The versatile nucleotide excision repair (NER) pathway initiates as the XPC–RAD23B–CETN2 complex first recognizes DNA lesions from the genomic DNA and recruits the general transcription factor complex, TFIIH, for subsequent lesion verification. Here, we present a cryo-EM structure of an NER initiation complex containing Rad4–Rad23-Rad33 (yeast homologue of XPC–RAD23B–CETN2) and 7-subunit coreTFIIH assembled on a carcinogen-DNA adduct lesion at 3.9–9.2 Å resolution. The coreTFIIH contains two helicase-family ATPase subunits: XPB(Ssl2) and XPD(Rad3) in human(yeast), and 5 nonenzymatic subunits: p62(Tfb1), p52(Tfb2), p44(Ssl1), p34(Tfb4), and p8(Tfb5). Altogether, our study illustrates how the Rad4–Rad23–Rad33 (XPC–RAD23B–CETN2) complex recruits TFIIH to damaged DNA in 3D structural models and provides the groundwork to visualize how the NER initiation is carried out in multiple, coordinated yet distinct steps.

The most populated class resolved TFIIH at a nominal resolution of 3.86 Å, but with disordered density corresponding to the Rad4–Rad23–Rad33 complex bound to DNA (Map 1, EMDB-22587). Map 1 resolved TFIIH at a nominal resolution of 3.86 Å, the highest resolution for yeast TFIIH so far reported. Local resolution calculations of Map 1 indicate that 6 of the 7 subunits of coreTFIIH (Rad3, Tfb1, Tfb2, Tfb4, Tfb5, and Ssl1) were determined at 3–6 Å resolution, whereas Ssl2 was determined at 6–8 Å resolution. Rad3 and its associated subunit Ssl1 were resolved at the highest resolution (~3–4 Å) within the complex. Within TFIIH, the structure of Ssl2 itself was a good match to the previous DNA-bound Ssl2 structures representing the characteristic pre-translocation state of this family of helicases/translocases although ATP could not be resolved in the catalytic site of Ssl241–43. In previous structures of TFIIH, the “open” form of Tfb5-Tfb2C (p52-p8 in humans) was stabilized by hydrophobic interactions between the N-terminal helix of Tfb5 (residues 14–26) and the adjacent hydrophobic helix (residues 563–571) of the Ssl2 C-terminal helicase domain (C-Ssl2, residues 549–776). In the TFIIH/Rad4–23–33/DNA complex, Tfb5-Tfb2C were rotated ~60° and stabilized in an alternative position (“closed” form). Compared with the previous structures of TFIIH, this Ssl2-Tfb5-Tfb2 made little contact with the rest of TFIIH, which allowed C-Ssl2 to move away from the rest of TFIIH by ~11 Å. The repositioning of Ssl2 relative to the rest of TFIIH is also consistent with the movement observed after multibody refinement of Map 1 that revealed a ~30° rotation of Ssl2-Tfb5-Tfb2C relative to the rest of TFIIH. Altogether, the current structures suggest that the rotation of Tfb5-Tfb2C and thereby unlocking Ssl2-Tfb5-Tfb2C from the rest of TFIIH may be key in stimulating the translocase activity of TFIIH (Ssl2) in an NER-specific manner.

> MKFYIDDLPVLFPYPKIYPEQYNYMCDIKKTLDVGGNSILEMPSGTGKTVSLLSLTIAYQMHYPEHRKIIYCSRTMSEIEKALVELENLMDYRTKELGYQEDFRGLGLTSRKNLCLHPEVSKERKGTVVDEKCRRMTNGQAKRKLEEDPEANVELCEYHENLYNIEVEDYLPKGVFSFEKLLKYCEEKTLCPYFIVRRMISLCNIIIYSYHYLLDPKIAERVSNEVSKDSIVIFDEAHNIDNVCIESLSLDLTTDALRRATRGANALDERISEVRKVDSQKLQDEYEKLVQGLHSADILTDQEEPFVETPVLPQDLLTEAIPGNIRRAEHFVSFLKRLIEYLKTRMKVLHVISETPKSFLQHLKQLTFIERKPLRFCSERLSLLVRTLEVTEVEDFTALKDIATFATLISTYEEGFLLIIEPYEIENAAVPNPIMRFTCLDASIAIKPVFERFSSVIITSGTISPLDMYPRMLNFKTVLQKSYAMTLAKKSFLPMIITKGSDQVAISSRFEIRNDPSIVRNYGSMLVEFAKITPDGMVVFFPSYLYMESIVSMWQTMGILDEVWKHKLILVETPDAQETSLALETYRKACSNGRGAILLSVARGKVSEGIDFDHQYGRTVLMIGIPFQYTESRILKARLEFMRENYRIRENDFLSFDAMRHAAQCLGRVLRGKDDYGVMVLADRRFSRKRSQLPKWIAQGLSDADLNLSTDMAISNTKQFLRTMAQPTDPKDQEGVSVWSYEDLIKHQNSRKDQGGFIENENKEGEQDEDEDEDIEMQ;> MSHSGAAIFEKVSGIIAINEDVSPAELTWRSTDGDKVHTVVLSTIDKLQATPASSEKMMLRLIGKVDESKKRKDNEGNEVVPKPQRHMFSFNNRTVMDNIKMTLQQIISRYKDADIYEEKRRREESAQHTETPMSSSSVTAGTPTPHLDTPQLNNGAPLINTAKLDDSLSKEKLLTNLKLQQSLLKGNKVLMKVFQETVINAGLPPSEFWSTRIPLLRAFALSTSQKVGPYNVLSTIKPVASSENKVNVNLSREKILNIFENYPIVKKAYTDNVPKNFKEPEFWARFFSSKLFRKLRGEKIMQNDRGDVIIDRYLTLDQEFDRKDDDMLLHPVKKIIDLDGNIQDDPVVRGNRPDFTMQPGVDINGNSDGTVDILKGMNRLSEKMIMALKNEYSRTNLQNKSNITNDEEDEDNDERNELKIDDLNESYKTNYAIIHLKRNAHEKTTDNDAKSSADSIKNADLKVSNQQMLQQLSLVMDNLINKLDLNQVVPNNEVSNKINKRVITAIKINAKQAKHNNVNSALGSFVDNTSQANELEVKSTLPIDLLESCRMLHTTCCEFLKHFYIHFQSGEQKQASTVKKLYNHLKDCIEKLNELFQDVLNGDGESMSNTCTAYLKPVLNSITLATHKYDEYFNEYNNNSN;> MSDYSLKHSVTQYLEEIPQQVQNRLYTSPATCLAIYRILPPLAKFFIMAMVFNENEVPLLDLDKWVNSNGKLQFQNAIKSMKSLHLLIPNKSSGTLMINLNPTFKISLRNALTGGEVQNSFGVVVEENVVSLDLLDEYSANKWETILHFMVGTPLAKIPSEKVLNLLKHSKLMEEVNSTGEFKITNEGFQFLLQEINSQLWTLLLQYLKMIETSKMDLVDVLHFIFMLGALEVGKAYKIDALSETQRIMLQDMRDYGLVFQKHSNDSIFYPTKLALMLTSDTKTIRSASNAMDSVLRQNREEPSVNEDGANGKSTTDITTSDDLNKAGLKNQDIPDGSLIVETNFKIYSYSNSPLQIAVLSLFVHLKARFVNMVLGQITRESIRRALTNGITADQIIAYLETHAHPQMRRLAEEKLEKKLELDPNCKEPLQVLPPTVVDQIRLWQLELDRVITYEGSLYSDFETSQEYNLLSKYAQDIGVLLWKDDKKKKFFISKEGNSQVLDFAKRKLKKKQ;> MDAISDPTFKHARSRKQVTEESPSLLTVIIEIAPKLWTTFDEEGNEKGSIIKVLEALIVFLNAHLAFNSANKVAVIAAYSQGIKYLYPESTSALKASESENKTRSDLKIINSDMYRRFRNVDETLVEEIYKLFELEKKQIEQNSQRSTLAGAMSAGLTYVNRISKESVTTSLKSRLLVLTCGSGSSKDEIFQYIPIMNCIFSATKMKCPIDVVKIGGSKESTFLQQTTDATNGVYLHVESTEGLIQYLATAMFIDPSLRPIIVKPNHGSVDFRTSCYLTGRVVAVGFICSVCLCVLSIIPPGNKCPACDSQFDEHVIAKLKRKPVVPRLKAKKKVTKP;> MARARKGALVQCDPSIKALILQIDAKMSDIVLEELDDTHLLVNPSKVEFVKHELNRLLSKNIYNPMDEEENQ;> MAPVVISESEEDEDRVAITRRTKRQVHFDGEGDDRVDQQQQQHSSSHRDRDKHVQRKKKKRLSNRNLQGSNGGYAWEDEIKRSWDLVKVDDEGDMASLVASIVEARKKRTAKKNITPYQRGIIRSLILTLDCSEAMLEKDLRPNRHAMIIQYAIDFVHEFFDQNPISQMGIIIMRNGLAQLVSQVSGNPQDHIDALKSIRKQEPKGNPSLQNALEMARGLLLPVPAHCTREVLIVFGSLSTTDPGDIHQTIDSLVSEKIRVKVLGLSAQVAICKELCKATNYGDESFYKILLDETHLKELFNEAVTPLPVNKINKGFTLVKMGFPTRIFEDTPTFCSCHSKLVYGGYFCPNCHSKVCSLPTVCPCCDLMLILSTHLARSYHHLMPLKTFAEVPTTEKFRSEDCFSCQSRFPILKNHKNGKLLTSSRYRCEDCKQEFCVDCDVFIHEILHNCPGCESKPVIT;> MTDVEGYQPKSKGKIFPDMGESFFSSDEDSPATDAEIDENYDDNRETSEGRGERDTGAMVTGLKKPRKKTKSSRHTAADSSMNQMDAKDKALLQDTNSDIPADFVPDSVSGMFRSHDFSYLRLRPDHASRPLWISPSDGRIILESFSPLAEQAQDFLVTIAEPISRPSHIHEYKITAYSLYAAVSVGLETDDIISVLDRLSKVPVAESIINFIKGATISYGKVKLVIKHNRYFVETTQADILQMLLNDSVIGPLRIDSDHQVQPPEDVLQQQLQQTAGKPATNVNPNDVEAVFSAVIGGDNEREEEDDDIDAVHSFEIANESVEVVKKRCQEIDYPVLEEYDFRNDHRNPDLDIDLKPSTQIRPYQEKSLSKMFGNGRARSGIIVLPCGAGKTLVGITAACTIKKSVIVLCTSSVSVMQWRQQFLQWCTLQPENCAVFTSDNKEMFQTESGLVVSTYSMVANTRNRSHDSQKVMDFLTGREWGFIILDEVHVVPAAMFRRVVSTIAAHAKLGLTATLVREDDKIGDLNFLIGPKLYEANWMELSQKGHIANVQCAEVWCPMTAEFYQEYLRETARKRMLLYIMNPTKFQACQFLIQYHERRGDKIIVFSDNVYALQEYALKMGKPFIYGSTPQQERMNILQNFQYNDQINTIFLSKVGDTSIDLPEATCLIQISSHYGSRRQEAQRLGRILRAKRRNDEGFNAFFYSLVSKDTQEMYYSTKRQAFLVDQGYAFKVITHLHGMENIPNLAYASPRERRELLQEVLLKNEEAAGIEVGDDADNSVGRGSNGHKRFKSKAVRGEGSLSGLAGGEDMAYMEYSTNKNKELKEHHPLIRKMYYKNLKK>MHHHHHHHMAVLTQAKIGDSLAEFLVEATPDPKLRQLMMSMAEATRTIAHKVRTASCAGTACVNSFGDEQLAVDMVADKLLFEALKYSHVCKLACSEEVPEPVDMGGEGFCVAFDPLDGSSIVDTNFAVGTIFGVWPGDKLTNITGREQVAAGMGIYGPRTVFCIALKDAPGCHEFLLMDDGKWMHVKETTHIGEGKMFAPGNLRATFDNPAYERLINFYLGEKYTLRYTGGMVPDVFQIIVKEKGVFTNVTSPTTKAKLRILFEVAPLALLIEKAGGASSCDGKAVSALDIPILVCDQRTQICYGSIGEVRRFEEY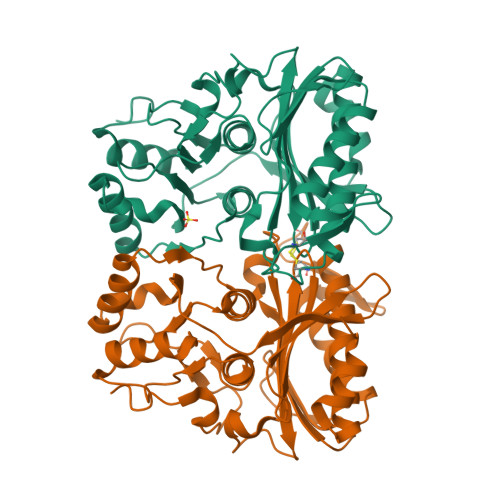MYGTSPRFSEKVAA[8x]>[3x]MEKTCIDALPLTMNSSEKQETVCIFGTGDFGRSLGLKMLQCGYSVVFGSRNPQKTTLLPSGAEVLSYSEAAKKSGIIIIAIHREHYDFLTELTEVLNGKILVDISNNLKINQYPESNAEYLAHLVPGAHVVKAFNTISAWALQSGALDASRQVFVCGNDSKAKQRVMDIVRNLGLTPMDQGSLMAAKEIEKYPLQLFPMWRFPFYLSAVLCVFLFFYCVIRDVIYPYVYEKKDNTFRMAISIPNRIFPITALTLLALVYLPGVIAAILQLYRGTKYRRFPDWLDHWMLCRKQLGLVALGFAFLHVLYTLVIPIRYYVRWRLGNLTVTQAILKKENPFSTSSAWLSDSYVALGILGFFLFVLLGITSLPSVSNAVNWREFRFVQSKLGYLTLILCTAHTLVYGGKRFLSPSNLRWYLPAAYVLGLIIPCTVLVIKFVLIMPCVDNTLTRIRQGWERNSKH

To gain insights into the molecular mechanisms that govern the metalloreductase activity of STEAP proteins, we determine structures of human STEAP4 using single-particle cryo-EM. The trimeric structures reveal an aligned, inter-subunit NADPH-FAD-heme arrangement and suggest that chelated iron(III) binds in a cavity of basic residues to facilitate reduction. Our biochemical and structural characterization of human STEAP4 elucidated that detergent-solubilized STEAP4 forms trimers that exhibit ferric-reductase activity in the presence of its redox cofactors, FAD and heme, and electron donor, NADPH, indicating that the enzyme does not require specific accessory proteins for catalysis. The trimeric arrangement observed in the cryo-EM structures is formed by interactions in STEAP protomers in both the OxRD and TMD layers, with a phospholipid molecule packed in between the TMDs of adjacent enzyme subunits, indicating that lipids stabilize the trimer.

We then determined structures of STEAP4EM in the presence of NADPH and FAD (cofactor-bound state) and in the presence of NADP+, FAD, and Fe3+-NTA (cofactor/substrate-bound state) using single-particle cryo-EM. The cofactor and cofactor/substrate-bound datasets yielded reconstructed density maps at 3.8 and 3.1 Å resolution, respectively. We argue that the difference in resolution is mainly caused by microscope type (200 kV FEI Arctica vs. 300 kV FEI Krios) and not by sample quality. The addition of cofactors NADPH and FAD, combined with lowering the pH from 8.0 to 5.5, strongly stabilized STEAP4EM and led to an increase in melting temperature of 11 °C (from 45.3 to 56.3 °C). Cryo-EM structures of STEAP4 in cofactor-bound and cofactor/substrate-bound states revealed the binding of FAD and heme molecules to the TMD of each protomer. At the intracellular side of the TMD cavity formed by helices h2–h5, we found density for an FAD molecule, which is axially anchored in the membrane through its tricyclic flavin ring. The adenine base stacks with W140 of a domain-swapped OxRD, indicating that FAD bridges the intracellular and TM domains of adjacent STEAP4 subunits. The shortest distance between FAD and heme is 9.6 Å. Although purified STEAP4EM displays catalytic activity, the nicotinamide ring of NADPH does not stack to a flavin ring in the observed structures; the closest flavin ring atom resides at ~18-Å distance in the adjacent STEAP4 TMD subunit. Binding of substrate Fe3+-NTA does not induce conformational rearrangements in STEAP4, because the densities of the cofactor/substrate and the cofactor-bound structures are virtually identical.5-{[(3beta,5beta,14beta,17alpha)-3-hydroxy-24-oxocholan-24-yl]amino}benzene-1,3-dicarboxylic acid 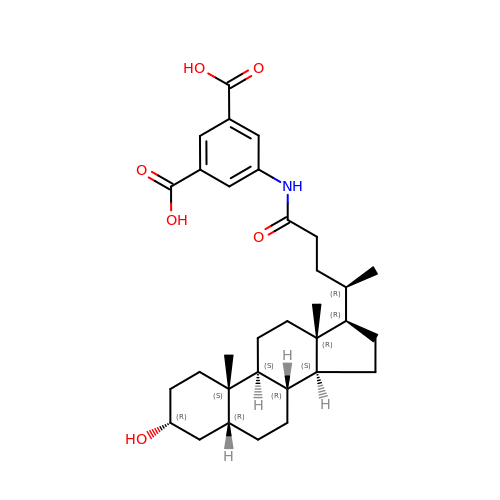| C32 H45 N O6 | BFYYXWCXPZTBMZ-ZCONXCDASA-N>[4x]MNKSQLYPDSPLTDQDFNQLDQTVIEAARRQLVGRRFIELYGPLGRGMQSVFNDIFMESHEAKMDFQGSFDTEVESSRRVNYTIPMLYKDFVLYWRDLEQSK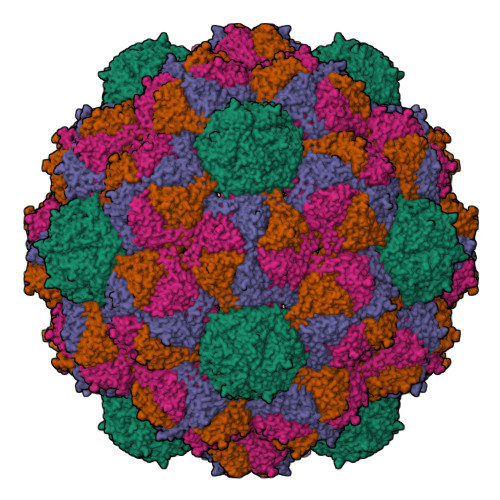ALDIPIDFSVAANAARDVAFLEDQMIFHGSKEFDIPGLMNVKGRLTHLIGNWYESGNAFQDIVEARNKLLEMNHNGPYALVLSPELYSLLHRVHKDTNVLEIEHVRELITAGVFQSPVLKGKSGVIVNTGRNNLDLAISEDFETAYLGEEGMNHPFRVYETVVLRIKRPAAICTLIDPEE;>[3x]TVGSLIQ> MSEMTPREIVSELDKHIIGQDNAKRSVAIALRNRWRRMQLNEELRHEVTPKNILMIGPTGVGKTEIARRLAKLANAPFIKVEATKFTEVGYVGKEVDSI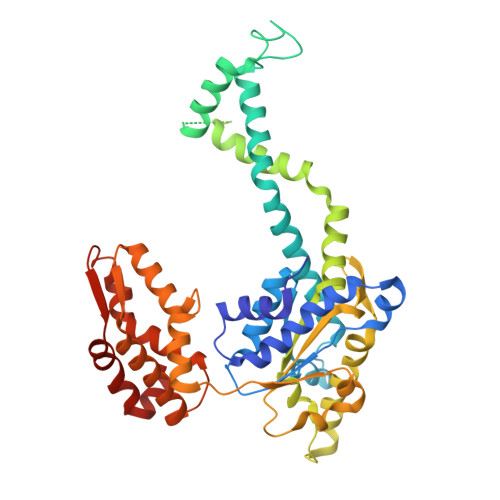IRDLTDAAVKMVRVQAIEKNRYRAEELAEERILDVLIPPAKNNWGQTEQQQEPSAARQAFRKKLREGQLDDKEIEIDLAAAPMGVEIMAPPGMEEMTSQLQSMFQNLGGQKQKARKLKIKDAMKLLIEEEAAKLVNPEELKQDAIDAVEQHGIVFIDEIDKICKRGESSGPDVSREGVQRDLLPLVEGCTVSTKHGMVKTDHILFIASGAFQIAKPSDLIPELQGRLPIRVELQALTTSDFERILTEPNASITVQYKALMATEGVNIEFTDSGIKRIAEAAWQVNESTENIGARRLHTVLERLMEEISYDASDLSGQNITIDADYVSKHLDALVADEDLSRFIL> ADRELEELLES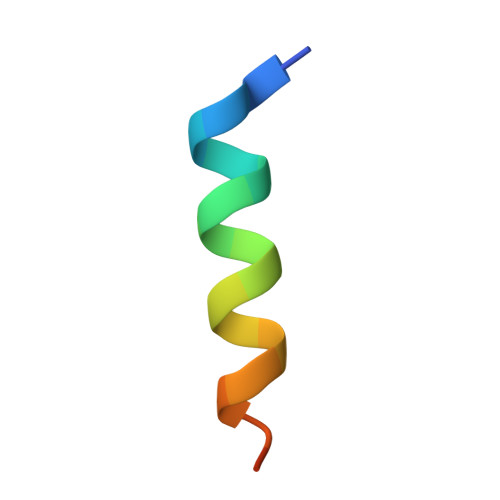ALDDFDKAK> GPHMKHPLMNVWTLWYLENDRSKSWEDMQNEITSFDTVEDFWSLYNHIKPPSEIKLGSDYSLFKKNIRPMWEDAANKQGGRWVITLNK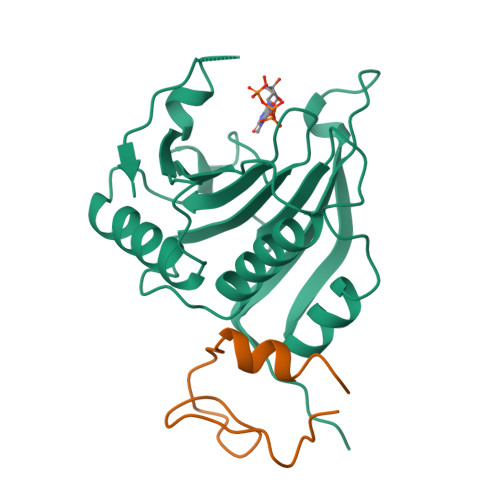SSKTDLDNLWLDVLLCLIGEAFDHSDQICGAVINIRGKSNKISIWTADGNNEEAALEIGHKLRDALRLGRNNSLQYQLHKDTMVKQGSNVKSIYTL;> GPHMSIINYNEGQWSPNNPSGKKQYDREQLLQLREVKASRIQPEVKNVSILPQPNLMPSFIRNN>WDQMCIEKEANKTYNCENLGLSEIPDTLPNTTEFLEFSFNFLPTIHNRTFSRLMNLTFLDLTRCQINWIHEDTFQSHHQLSTLVLTGNPLIFMAETSLNGPKSLKHLFLIQTGISNLEFIPVHNLENLESLYLGSNHISSIKFPKDFPARNLKVLDFQNNAIHYISREDMRSLEQAINLSLNFNGNNVKGIELGAFDSTIFQSLNFGGTPNLSVIFNGLQNSTTQSLWLGTFEDIDDEDISSAMLKGLCEMSVESLNLQEHRFSDISSTTFQCFTQLQELDLTATHLKGLPSGMKGLNLLKKLVLSVNHFDQLCQISAANFPSLTHLYIRGNVKKLHLGVGCLEKLGNLQTLDLSHNDIEASDCCSLQLKNLSHLQTLNLSHNEPLGLQSQAFKECPQLELLDLAFTRLHINAPQSPFQNLHFLQVLNLTYCFLDTSNQHLLAGLPVLRHLNLKGNHFQDGTITKTNLLQTVGSLEVLILSSCGLLSIDQQAFHSLGKMSHVDLSHNSLTCDSIDSLSHLKGIYLNLAANSINIISPRLLPILSQQSTINLSHNPLDCTCSNIHFLTWYKENLHKLEGSEETTCANPPSLRGVKLSDVKLSCG[2x];>GGGGKAWPTHVVCSDSGLEVLYQSCDPLQDFGFSVEKCSKQLKSNINIRFGIILREDIKELFLDLALMSQGSSVLNFSYPICEAALPKFSFCGRRKGEQIYYAGPVNNPEFTIPQGEYQVLLELYTE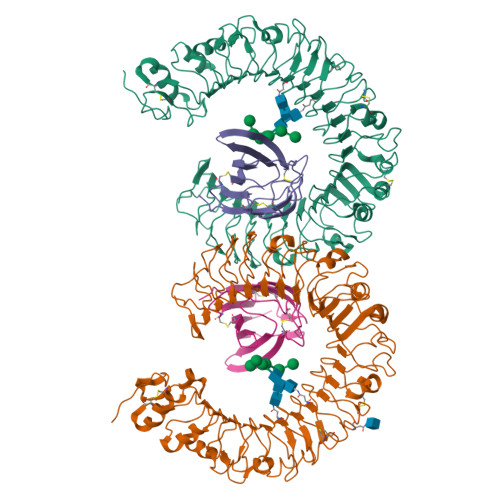KRSTVACANATIMCSEF[2x]>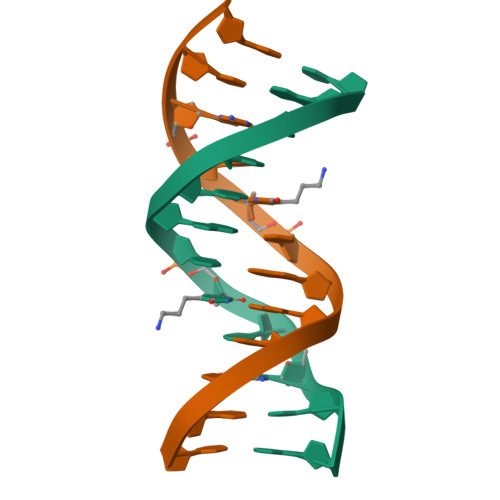CGCGAATUCGCG[2x]> XSSLSPTEGKGSGLQGHIIENPQYFSDACVHHIKRRDI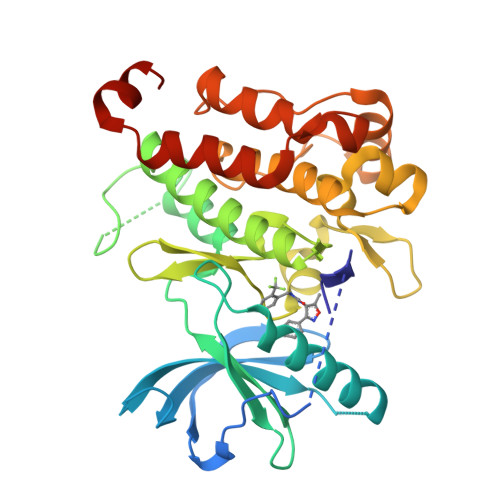VLKWELGEGAFGKVFLAECHNLLPEQDKMLVAVKALKEASESARQDFQREAELLTMLQHQHIVRFFGVCTEGRPLLMVFEYMRHGDLNRFLRSHGPDAKLLAGGEDVAPGPLGLGQLLAVASQVAAGMVYLAGLHFVHRDLATRNCLVGQGLVVKIGDFGMSRDIYSTDYYRVGGRTMLPIRWMPPESILYRKFTTESDVWSFGVVLWEIFTYGKQPWYQLSNTEAIDCITQGRELERPRACPPEVYAIMRGCWQREPQQRHSIKDVHARLQALAQAPPVYLDVLGHHHHHH>[20x]MGRGKVKPNRKSTGDNSNVVTMIRAGSYPKVNPTPTWVRAIPFEVSVQSGIA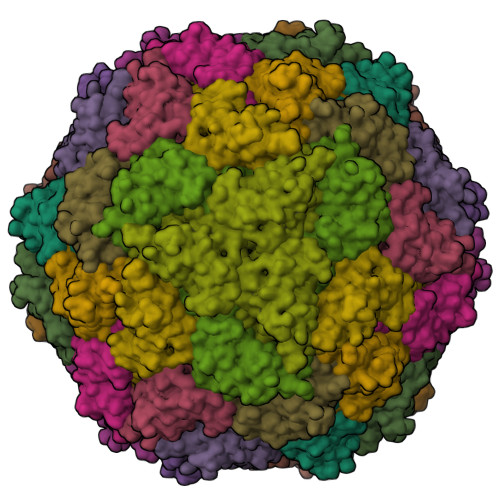FKVPVGSLFSANFRTDSFTSVTVMSVRAWTQLTPPVNEYSFVRLKPLFKTGDSTEEFEGRASNINTRASVGYRIPTNLRQNTVAADNVCEVRSNCRQVALVISCCFN Protein stability can be fine‐tuned by modifying different structural features such as hydrogen‐bond networks, salt bridges, hydrophobic cores, or disulfide bridges. Among these, stabilization by salt bridges is a major challenge in protein design and engineering since their stabilizing effects show a high dependence on the structural environment in the protein, and therefore are difficult to predict and model. In this work, we explore the effects on structure and stability of an introduced salt bridge cluster in the context of three different de novo TIM barrels. The results show that despite the similarities in protein fold, the salt bridge clusters differently influence the structural and stability properties of the de novo TIM barrel variants depending on the structural background where they are introduced.

The salt bridge variants exhibit similar thermostability in comparison with their parental designs but important differences in the conformational stability at 25°C can be observed such as a highly stabilizing effect for two of the proteins but a destabilizing effect to the third. Analysis of the formed geometries of the salt bridge cluster in the crystal structures show either highly ordered salt bridge clusters or only single salt bridges. Rosetta modeling of the salt bridge clusters results in a good prediction of the tendency on stability changes but not the geometries observed in the three‐dimensional structures.

> MDKDEAWKQVEILRRLGAKRIAYRSDDWRDLQEALKKGADILIVDATDKDEAWKQVEILRRLGAKEIAYRSDDWRDLQEALKKGADILIVDATDKDEAWKQVEILRRLGAKRIAYRSDDWRDLQEALKKGADILIVDATDKDEAWKQVEILRRLGAKEIAYRSDDWRDLQEALKKGADILIVDATGLEHHHHHH(1,8-DIHYDROXY-9-OXO-9,10-DIHYDRO-ANTHRACEN-2-YL)-ACETIC ACID | C16 H12 O5 | 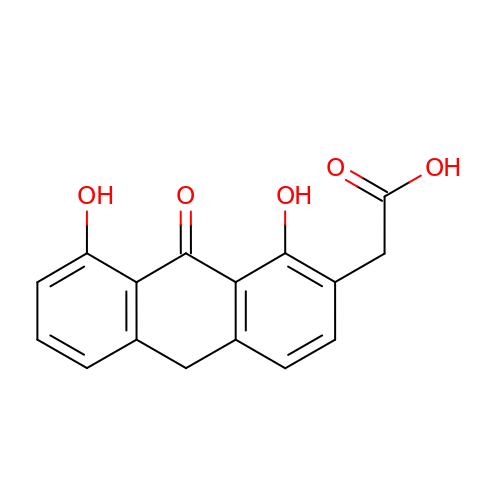IXLRLZOYKJERRA-UHFFFAOYSA-N>[2x]MWSHPQFEKGGSGNSGQNLENIKKFIRAANYLTVSQIFLQDNFLLERPLTFEDIKPRLLGHWGSCPGVNWVYAHLLNIQKQLEFAKSGLKAAFMLGPGHAFPALQANLFMEETLSKVDKKATRNAQGIEYISKNFSWPGGFPSSASPFTPGVILEGGELGYSLSTAFGAILDNPNLVMTTLIGDGEAETGSIAAAWHLSKLIDPVKNGVVLPVLHLNGYKISGPTIFGSMSDFELIQFFHGAGWEPKIVDEYSAEDFDLELSNAFSNAFRDISRIKFGRNSKFIRLPMIIMRSKKGSSGVKENNGQKIEGNSLAHQVPLLKAKTDKNELEKLENWMKSYKFDELFDYERGEFKWWINDFLPENSSRIGRNRFVDANLNFKELKLPEITEGFGEKSLAMNAVGSLLE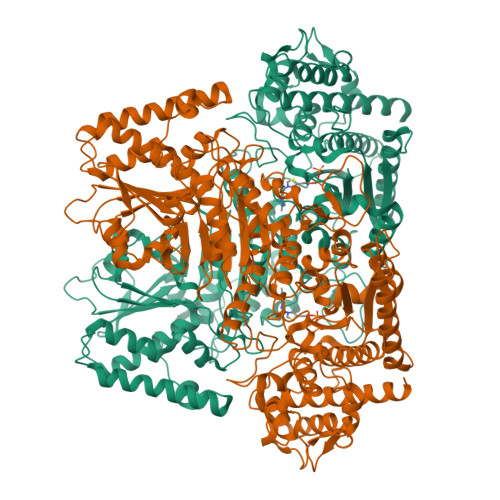KVFEKNPDNFRFFSPDETYSNKLDAIFEATSRSWQREIKPWEKDLAKNGRVTEILSENCLQGLLQGYILTGRYGVLTSYEAFAPVISSMMDQYAKFLAQSKEVKWRGDLASLNYILTSTGWRQDHNGFNHQNPSFIDEVLRRENGIGQIFLPADDNSAVAAISKMLKTRNNINVLVAGKTPEPRYFSLESAQKQLENGGIFVFDSWKNQKITDWDSISEDDEPDLILAASGDYVFKETVAALQVLLHDVAQVKIRLVYIQALCGKGIGTFENTLSKSDFVKIFTKDKPVIFAFHGYAKTLKSILFDYENPARIQINGYEEKGSTTTPFDMLARNKVSRYDITVRALKSVSEGDKVFGSLVKEYRKRQDDALRFAQENSVDAPEIENWDYLRFF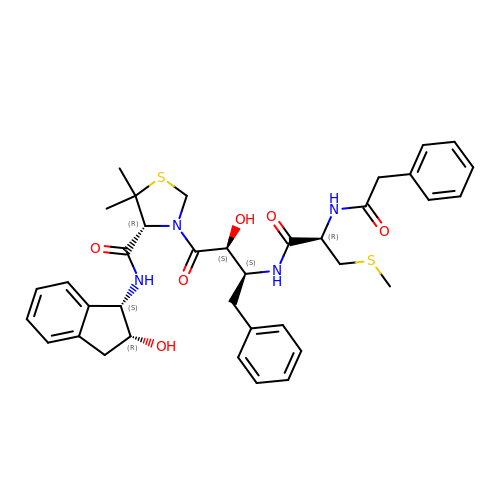(4R)-N-[(1S,2R)-2-hydroxy-2,3-dihydro-1H-inden-1-yl]-3-[(2S,3S)-2-hydroxy-3-{[S-methyl-N-(phenylacetyl)-L-cysteinyl]amino}-4-phenylbutanoyl]-5,5-dimethyl-1,3-thiazolidine-4-carboxamide | C37 H44 N4 O6 S2 | FCTXMHJXDHGIIN-ACUZRORGSA-N> G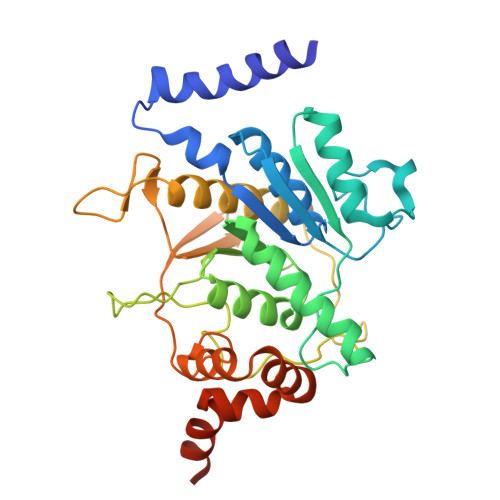PHMLKIADQSVDLNLKLMKWRILPDLNLDIIKNTKVLLLGAGTLGCYVSRALIAWGVRKITFVDNGTVSYSNPVRQALYNFEDCGKPKAELAAASLKRIFPLMDATGVKLSIPMIGHKLVNEEAQHKDFDRLRALIKEHDIIFLLVDSRESRWLPSLLSNIENKTVINAALGFDSYLVMRHGNRDEQSSKQLGCYFCHDVVAPTDSLTDRTLDQMCTVTRPGVAMMASSLAVELMTSLLQTKYSGSETTVLGDIPHQIRGFLHNFSILKLETPAYEHCPACSPKVIEAFTDLGWEFVKKALEHPLYLEEISGLSVIKQEVERLGNDVFEWEDDESDEIA> GSSVVVDTNGQPVSNGADAYYLVPVSHGHAGLALAKIGNEAEPRAVVLDPHHRPGLPVRFESPLRINIIKESYFLNIKFGPSSSDSGVWDVI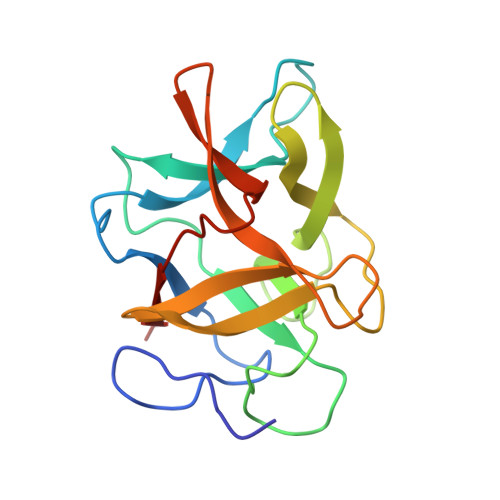QQDPIGLAVKVTDTKSLLGPFKVEKEGEGYKIVYYPERGQTGLDIGLVHRNDKYYLAVKDGEPCVFKIRKAT>MSETSRTAFGGRRAVPPNNSNAAEDDLPTVELQGVVPRGVNLQEFLNVTSVHLFKERWDTNKVDHHTDKYENNKLIVRRGQSFYVQIDFSRPYDPRRDLFRVEYVIGRYPQENKGTYIPVPIVSELQSGKWGAKIVMREDRSVRLSIQSSPKCIVGKFRMYVAVWTPYGVLRTSRNPETDTYILFNPWCEDDAVYLDNEKEREEYVLNDIGVIFYGEVNDIKTRSWSYGQFEDGILDTCLYVMDRAQMDLSGRGNPIKVSRVGSAMVNAKDDEGVLVGSWDNIYAYGVPPSAWTGSVDILLEYRSSENPVRYGQCWVFAGVFNTFLRCLGIPARIVTNYFSAHDNDANLQMDIFLEEDGNVNSKLTKDSVWNYHCWNEAWMTRPDLPVGFGGWQAVDSTPQENSDGMYRCGPASVQAIKHGHVCFQFDAPFVFAEVNSDLIYITAKKDGTHVVENVDATHIGKLIVTKQIGGDGMMDITDTYKFQEGQEEERLALETALMYGAKKPLNTEGVMKSRSNVDMDFEVENAVLGKDFKLSITFRNNSHNRYTITAYLSANITFYTGVPKAEFKKETFDVTLEPLSFKKEAVLIQAGEYMGQLLEQASLHFFVTARINETRDVLAKQKSTVLTIPEIIIKVRGTQVVGSDMTVTVEFTNPLKETLRNVWVHLDGPGVTRPMKKMFREIRPNSTVQWEEVCRPWVSGHRKLIASMSSDSLRHVYGELDVQIQRRPSM[2x];>[2x]MRLKNLTFIIILIISGELYAEEKPCGFPHVENGRIAQYYYTFKSFYFPMSIDKKLSFFCLAGYTTESGRQEEQTTCTTEGWSPEPRCFKKCTKPDLSNGYISDVKLLYKIQENMRYGCASGYKTTGGKDEEVVQCLSDGWSSQPTCRKEHETCLAPELYNGNYSTTQKTFKVKDKVQYECATGYYTAGGKKTEEVECLTYGWSLTPKCTKLKCSSLRLIENGYFHPVKQTYEEGDVVQFFCHENYYLSGSDLIQCYNFGWYPESPVCEGRRNRCPPPPLPINSKIQTHSTTYRHGEIVHIECELNFEIHGSAEIRCEDGKWTEPPKCIEGQEKVACEEPPFIENGAANLHSKIYYNGDKVTYACKSGYLLHGSNEITCNRGKWTLPPECVENNENCKHPPVVMNGAVADGILASYATGSSVEYRCNEYYLLRGSKISRCEQGKWSSPPVCLEPCTVNVDYMNRNNIEMKWKYEGKVLHGDLIDFVCKQGYDLSPLTPLSELSVQCNRGEVKYPLCTRKES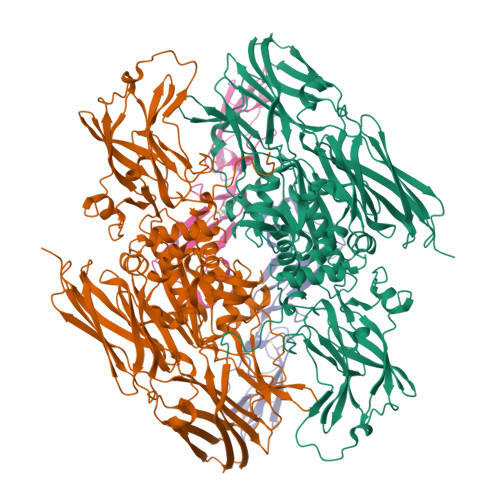KGMCTSPPLIKHGVIISSTVDTYENGSSVEYRCFDHHFLEGSREAYCLDGMWTTPPLCLEPCTLSFTEMEKNNLLLKWDFDNRPHILHGEYIEFICRGDTYPAELYITGSILRMQCDRGQLKYPRCIPRQSTLSYQEPLRT(3S,4R)-N-[2-chloro-5-(2-methoxyethyl)benzyl]-N-cyclopropyl-4-{6-[2-(2,6-dichloro-4-methylphenoxy)ethoxy]pyridin-3-yl}-4-hydroxypiperidine-3-carboxamide | C33 H38 Cl3 N3 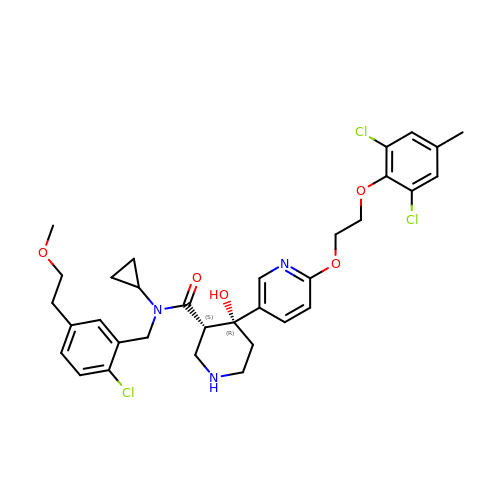O5 | ACRSSIRQZLKXJN-NYFMKLKXSA-N>WVPHELTENQKNRRFEVSSSLILRNHNEPFLDRIVTCDEKWILYDNRRRSAQWLDQEEAPKHFPKPILHPKKVMVTIWWSAAGLIHYSFLNPGETITSEKYAQEIDEMNQKLQRLQLALVNRKGPILLHDNARPHVAQPTLQKLNELGYEVLPHPPYSPDLLPTNYH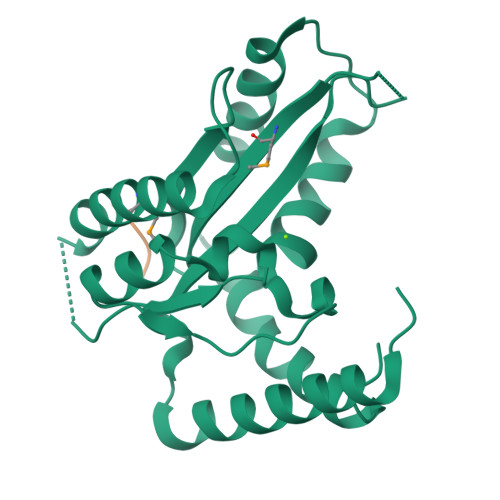VFKHLNNFLQGKRFHNQQDAENAFQEFVESQSTDFYATGINQLISRWQKCVDCNGSYFD[2x];> LYFA> MGHSSSDPVYPCGICTNEVNDDQDAILCEASCQKFFHRICTGMTETAYGLLTAEASAVWGCDTCMADKDVQ;> AAKVVYVFSTEMANKAAEAVLKGQVETIVSFHI

Pygo and BCL9/Legless transduce the Wnt signal by promoting the transcriptional activity of β-catenin/Armadillo in normal and malignant cells. Molecularly, BCL9/Lgs proteins function as adaptors between Pygo and Armadillo/β-catenin, by binding through their homology domain 1 (HD1) to the PHD finger in the C terminus of Pygo, and through their homology domain 2 (HD2) to the Armadillo repeat domain of Armadillo/β-catenin (Kramps et al., 2002; Städeli and Basler, 2005). We show that human and Drosophila Pygo PHD fingers associate with their cognate HD1 domains from BCL9/Legless to bind specifically to the histone H3 tail methylated at lysine 4 (H3K4me). Therefore, this is a prime example of histone tail binding by a PHD finger (of Pygo) being modulated by a cofactor (BCL9/Legless).

Here, we report the crystal structure of the human PHD-HD1 complex. Our structures of the PHD-HD1 complex identify the PHD loop2 segment as the BCL9-interacting surface, with a relatively flat and hydrophobic nature. The interaction has two parts, a parallel β sheet between strands PHD β5 and HD1 β1, and a hydrophobic core between the two helices. The buried surface area is relatively small (∼1240 Å2, 15% and 18% of the total solvent-accessible surface areas of PHD and HD1, respectively), which is consistent with a relatively transient interaction, as might be expected for a signaling molecule. Superimposition of our structures of the PHD-HD1 complex on that of the free hPHD finger (Nakamura et al., 2007) shows that the structures are very similar (rmsd for the Cα backbone, 0.6 Å), except for small local conformational changes of two short loop segments. The second difference is in the PHD-HD1 interface, in a loop segment between α1 and β5 (L382–S387). This loop is pushed out in the binary complex compared to the free PHD finger (arrow 2), as a direct consequence of the PHD-HD1 interactions, opening up the A1 cavity in the complex.> SLKRLAFSSLSHTLAPFPEGELDAHLSDADFTRVFTEEDDLDLVAQSLPLVLKVYEALHLQNPAHRGLSLAVGRLYIMYANAFVQTPAQYLPEDEFEAQNEAYSRARKLYLRGARYALSSLETAYPGFTREVFSGDEQRLHKVLSRCTRVDVGTLYWVGTGYVAAFALTPLGSALPDTVHAAVMMLERACDLWPSYQEGAVWNVLTKFYAAAPESFGGGMEKAHTAFEHLTRYCSAHDPDHHITYADALCIPLNNRAGFDEALDRALAIDPESVPH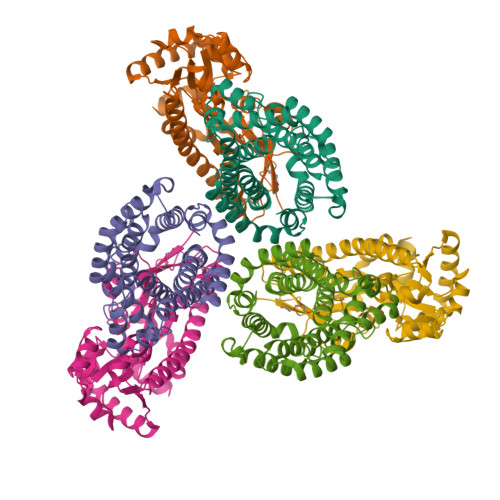NKLLVILSQKRARWLKAHVQDFFLD;> GRKEKVVLKIASIAPARSIWETELKKLSAEWSEITGGLVSMKFYDMSSLGGEREGIRKLKSSRPGQAAPLDGAVFSCLGLSELAPDSGIYTLSVPFLIQNEKDLERVLHELREDLDRPFRAAGFRVITWTNAGWLSFYTRAPYASLGQLKKQTIALSSLDSSVLGTCFRICGFDIKDAPNVRLAPLLKAGSIDGFLSVHLFTWATGFYRYISYALDTKICPAVIGMLISDGSWARIPSRYHDAMLQAATRVRQRLANNLETLDRECSNNIQKAGVSIVHLTPQEIQEWRTEFAADVKRIQARLPGMLNMTLYEKIKHLLYSAQR>DREIKEEARKLIREAIELLQKGDPRAKEILRQAILILLAIRLLEEMEENIEKAEKLGNEELSELAKRAIKLVREALELLKEGDPRAEEILKLALKIIKAILLLLEMYENIKQAEELGDEDLSELAKIAIRLVRQALKLLQEGDPRAEE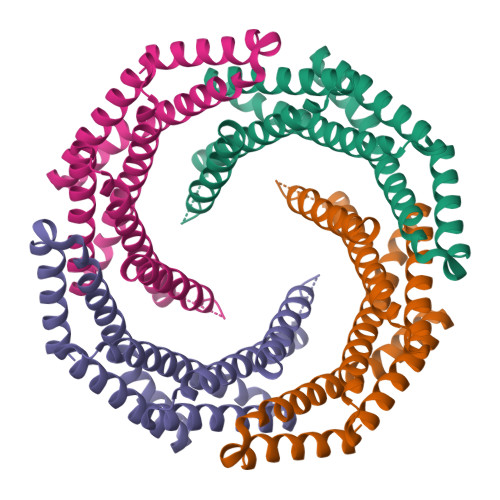ILEIALRIIKLILQLLFLKQRIEEAKKKGDQQFVFEAEEKIRRIVEELFKLLEG[4x]>[11x]GSMKKVEAIIRPEKLEIVKKALSDAGYVGMTVSEVKGRGVQGGIVERYRGREYIVDLIPKVKIELVVKEEDVDNVIDIICENART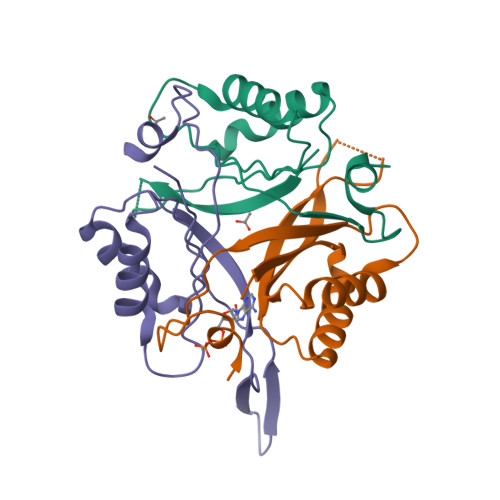GNPGDGKIFVIPVERVVRVRTKEEGKEALLEHHH;> GSMKKVEAIIRPEKLEIVKKALSDAGYVGMTVSEVKGRGVQGGIVERYRGREYIVDLIPKVKIELVVKEEDVDNVIDIICENARTGNPGDGKIFVIPVERVVRVRTKEEGKEALEEHHH> SMGGTHIDLLFHPPRAHLLTIKETIRKMIKEARKVIALVMDIFTDVDIFKEIVEASTRGVSVYILLDESNFNHFLNMTEKQGCSVQRLRNIRVRTVKGQDYLSKTGAKFHGKMEQKFLLVDCQKVMYGSYSYMWSFEKAHLSMVQIITGQL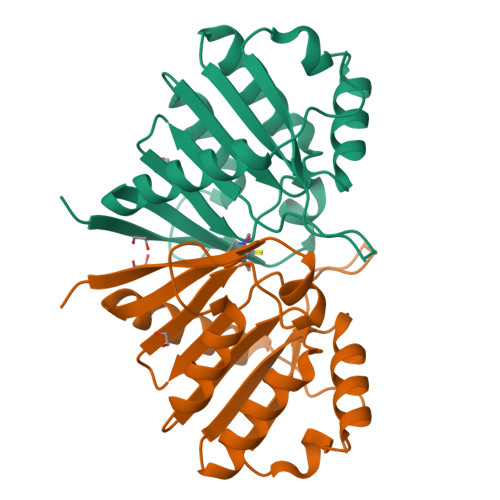VESFDEEFRTLYARSCVPSSFAQEESARV Inosine-5′-monophosphate dehydrogenase (IMPDH) catalyzes the rate-limiting oxidation of IMP to xanthosine 5′-monophosphate (XMP) in the pathway of guanine nucleotide synthesis and is thus a key player in the regulation of the intracellular purine nucleotide pools of almost every organism. Although mammalian cells synthesize purine nucleotides de novo, T. brucei is auxotrophic for purines and critically depends on salvage mechanisms, including the IMPDH-catalyzed reaction, to acquire these nucleotides from the extracellular environment. Recent evidences indicate that the activity of the catalytic domain of IMPDH is allosterically controlled by a nucleotide-mediated regulatory switch. Combining recombinant in cellulo protein crystallization and serial femtosecond crystallography (SFX), we here present the structure of IMPDH from Trypanosoma brucei.

In cellulo grown crystals of TbIMPDH isolated from baculovirus-infected Sf9 insect cells diffracted up to 2.80 Å resolution, exploiting the 40-fs X-ray pulses of the X-ray free-electron laser (XFEL) Linac Coherent Light Source (LCLS) at the CXI beamline. The crystals belonged to the space group P4 21 2 containing two TbIMPDH monomers in the asymmetric unit (ASU), corresponding to ~75% solvent in the crystal lattice. Extra electron density was identified in two clefts on the surface of the Bateman domain that were unambiguously assigned to one ATP molecule and one GMP molecule. However, instead of GDP or GTP, GMP occupies the second canonical site in TbIMPDH, exhibiting a flipped, so far unknown nucleotide coordination mode for Bateman domains. This enables the formation of direct interactions with the catalytic domain, resulting in a stabilization of the compact IMPDH oligomer conformation. As a consequence of the observed flipped binding mode, an interaction of the two bound nucleotides in the canonical sites via Mg2+ ions, coordinating two ATPs, as described by Labesse et al. and Buey et al. for A. gossypii and P. aeruginosa IMPDHs, is prevented. If guanine nucleotides bind to the second canonical site of the Bateman domain, a more closed angle was previously reported (e.g. 125° in AgIMPDH-GDP1/GDP2/GDP3), compared to the corresponding ATP complexes (e.g. 155° in AgIMPDH-ATP1/ATP2). This is confirmed for TbIMPDH-ATP1/GMP2, exhibiting a bending angle of ~115°. However, the TbIMPDH structure clearly reveals guanine nucleotide specificity for the second canonical site in a quasi-physiological environment of the enzyme.

>[2x]MENTNLRTKTLRDGTTAEELFSQDGLSFNDFIILPGFIDFDSSKVNVSGQFTKNILLHLPLVSSPMDTVTESSMARAMALMGGIGVIHNNCTVEQQARMVRSVKLYRNGFIMKPKSVSPDVPVSTIRNIKSEKGISGILVTEGGKYDGKLLGIVCTKDIDFVKDASAPVSQYMTRRENMTVERYPIKLEEAMDVLNRSRHGYLPVLNDKDEVVCLCSRRDAVRARDYPNSSLDRNGHLLCAAATSTREADKGRVAALSEAGIDVLVLDSSQGNTIYQVSFIRWVKKTYPHLEVVAGNVVTQDQAKNLIDAGADSLRIGMGSGSICITQEVLACGRPQATAIYKVARYAASRGVPCVADGGLRNVGDVCKALAVGANVAMLGSMIAGTSETPGEYFFKDGMRLKGYRGMGSIDAMLQGRESGKRYLSENETLQVAQGVAGAVLDKGSVLKLLAYIHKGLQQSAQDIGEVSFDAIREKVYEGQVLFNRRTLTAQSEGAVHSLHHYERKLFASKL> MKLEINKFNYNDPIDGINVITMRPPRHSDKINKGKGPFKAFQVIKNIWIVPERYNFTNNTNDLNIPSEPIMEADAIYNPNYLNTPSEKDEFLQGVIKVLERIKSKPEGEKLLELISSSIPLPLVSNGALTLSDNETIAYQENNNIVSNLQANLVIYGPGPDIANNATYGLYSTPISNGEGTLSEVSFSPFYLKPFDESYGNYRSLVNIVNKFVKREFAPDPASTLMHELVHVTHNLYGISNRNFYYNFDTGKIETSRQQNS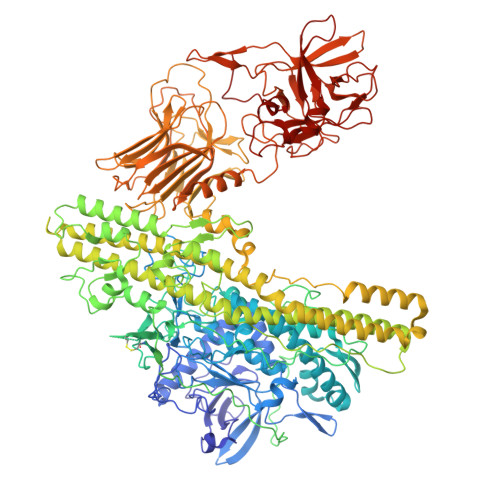LIFEELLTFGGIDSKAISSLIIKKIIETAKNNYTTLISERLNTVTVENDLLKYIKNKIPVQGRLGNFKLDTAEFEKKLNTILFVLNESNLAQRFSILVAKHFLKERPIDPIYVNILDDNSYSTLEGFNISSQGSNDFQGQLLESSYFEKIESNALRAFIKICPRNGLLYNAIYRNSKNYLNNIDLEDKKTTSKTNVSYPCSLLNGCIEVENKDLFLISNKDSLNDINLSEEKIKPETTVFFKDKLPPQDITLSNYDFTEANSIPSISQQNILERNEELYEPIRNSLFEIKTIYVDKLTTFHFLEAQNIDESIDSSKIRVELTDSVDEALSNPNKVYSPFKNMSNTINSIETGITSTYIFYQWLRSIVKDFSDETGKIDVIDKSSDTLAIVPYIGPLLNIGNDIRHGDFVGAIELAGITALLEYVPEFTIPILVGLEVIGGELAREQVEAIVNNALDKRDQKWAEVYNITKAQWWGTIHLQINTRLAHTYKALSRQANAIKMNMEFQLANYKGNIDDKAKIKNAISETEILLNKSVEQAMKNTEKFMIKLSNSYLTKEMIPKVQDNLKNFDLETKKTLDKFIKEKEDILGTNLSSSLRRKVSIRLNKNIAFDINDIPFSEFDDLINQYKNEIEDYEVLNLGAEDGKIKDLSGTTSDINIGSDIELADGRENKAIKIKGSENSTIKIAMNKYLRFSATDNFSISFWIKHPKPTNLLNNGIEYTLVENFNQRGWKISIQDSKLIWYLRDHNNSIKIVTPDYIAFNGWNLITITNNRSKGSIVYVNGSKIEEKDISSIWNTEVDDPIIFRLKNNRDTQAFTLLDQFSIYRKELNQNEVVKLYNYYFNSNYIRDIWGNPLQYNKKYYLQTQDKPGKGLIREYWSSFGYDYVILSDSKTITFPNNIRYGALYNGSKVLIKNSKKLDGLVRNKDFIQLEIDGYNMGISADRFNEDTNYIGTTYGTTHDLTTDFEIIQRQEKYRNYCQLKTPYNIFHKSGLMSTETSKPTFHDYRDWVYSSAWYFQNYENLNLRKHTKTNWYFIPKDEGWDED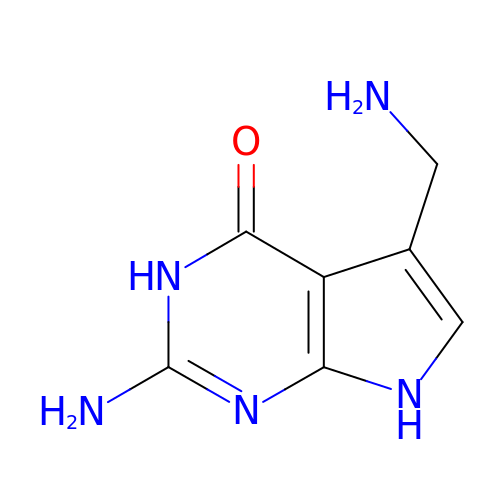7-DEAZA-7-AMINOMETHYL-GUANINE | C7 H9 N5 O | MEYMBLGOKYDGLZ-UHFFFAOYSA-N7-[(3-aminopropyl)amino]-1-sulfanylheptan-2-one 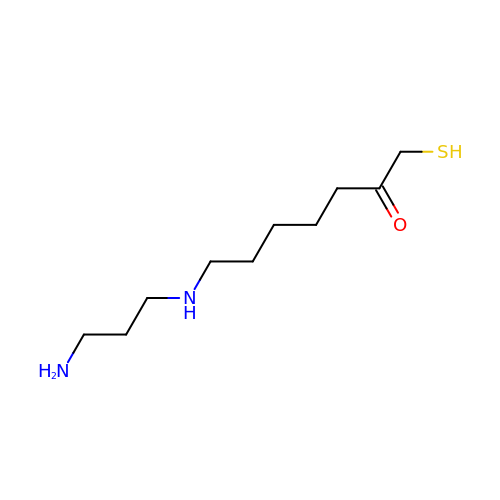| C10 H22 N2 O S | OOZNPNMKAJIVIZ-UHFFFAOYSA-N>MTVTYTARVANARFGGFSQLLLLWRGSIYKLLWRELLCFLGFYMALSAAYRFVLTEGQKRYFEKLVIYCDQYASLIPVSFVLGFYVTLVVNRWWSQYLCMPLPDALMCVVAGTVHGRDDRGRLYRRTLMRYAGLSAVLILRSVSTAVFKRFPTIDHVVEAGFMTREERKKFENLNSSYNKYWVPCVWFSNLAAQARREGRIRDNSALKLLLEELNVFRGKCGMLFHYDWISVPLVYTQVVTIALYSYFLACLIGRQFLDPAQGYKDHDLDLCVPIFTLLQFFFYAGWLKVAEQLINPFGEDDDDFETNFLIDRNFQVSMLAVDEMYDDLAVLEKDLYWDAAEARAPYTAAT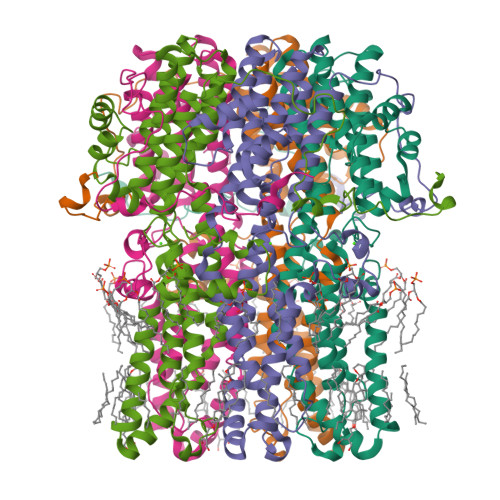VFQLRQPSFQGSTFDITLAKEDMQFQRLDGLDGPMGEAPGDFLQRLLPAGAGMVA[5x]> SMSLPKVMIVVGGQAPKAIRSVECYDFEEDRWDQIAELPSRRCRAGVVFMAGHVYAVGGFNGSLRVRTVDVYDGVKDQWTS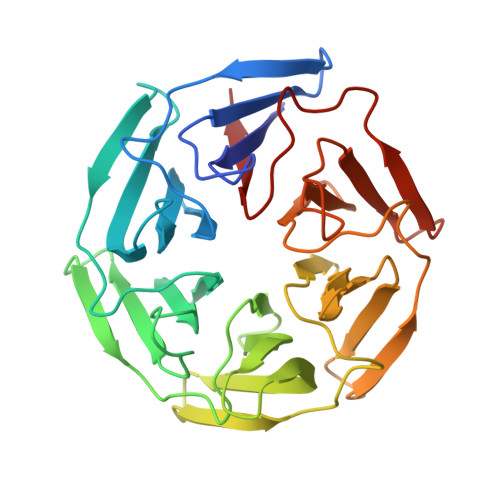IASMQERRSTLGAAVLNDLLYAVGGFDGSTGLASVEAYSYKTNEWFFVAPMNTRRSSVGVGVVEGKLYAVGGYDGASRQCLSTVEQYNPATNEWIYVADMSTRRSGAGVGVLSGQLYATGGHDGPLVRKSVEVYDPGTNTWKQVADMNMCRRNAGVCAVNGLLYVVGGDDGSCNLASVEYYNPVTDKWTLLPTNMSTGRSYAGVAVIHKSL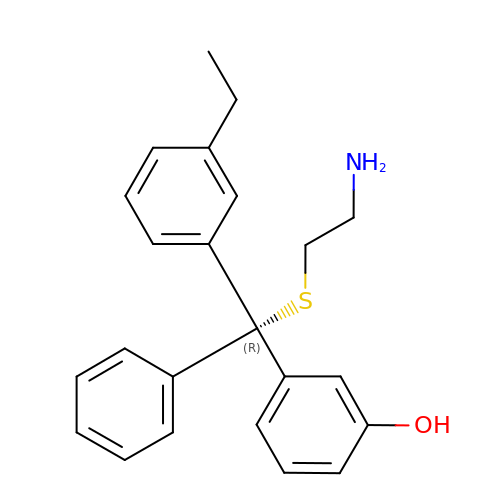3-[(R)-2-azanylethylsulfanyl-(3-ethylphenyl)-phenyl-methyl]phenol | C23 H25 N O S | LKEJFEOGGYEWTI-HSZRJFAPSA-N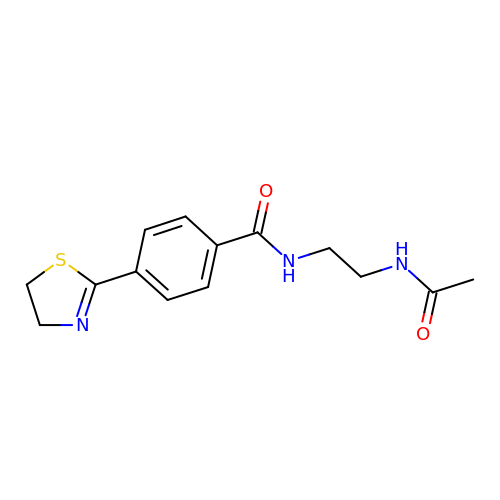N-(2-acetamidoethyl)-4-(4,5-dihydro-1,3-thiazol-2-yl)benzamide | C14 H17 N3 O2 S | RTMXZJKKASUKFJ-UHFFFAOYSA-N> GHMGSSGGCTSMMNLVLCFTGFRKKEELVRLVTLVHHMGGVIRKDFNSKVTHLVANCTQGEKFRVAVSLGTPIMKPEWIYKAWERRNEQDFYAAVDDFRNEFKVPPFQDCILSFLGFSDEEKTNMEEMTEMQGGKYLPLGDERCTHLVVEENIVKDLPFEPSKKLYVVKQEWFWGSIQMDARAGETMYLYEKANTPELKKSVSMLSLNTPNSNRKRRRLKETLAQLSRETDVSPFPPRKRPSAEHSLSIGSLLDISNT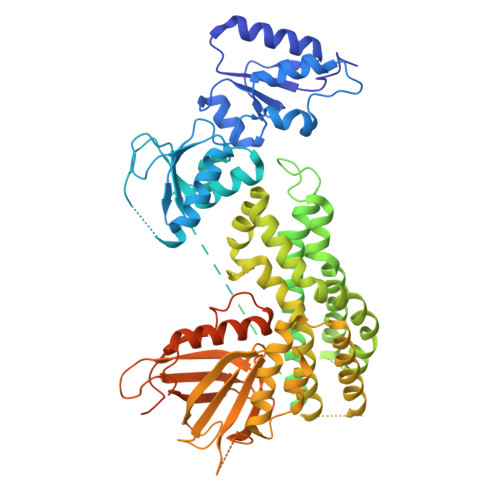PESSINYGDTPKSCTKSSKSSTPVPSKQSARWQVAKELYQTESNYVNILATIIQLFQVPLEEEGQRGGPILAPEEIKTIFGSIPDIFDVHTKIKDDLEDLIVNWDESKSIGDIFLKYSKDLVKTYPPFVNFFEMSKETIIKCEKQKPRFHAFLKINQAKPECGRQSLVELLIRPVQRLPSVALLLNDLKKHTADENPDKSTLEKAIGSLKEVMTHINEDKRKTEAQKQIFDVVYEVDGCPANLLSSHRSLVQRVETISLGEHPCDRGEQVTLFLFNDCLEIARKRHKVIGTFRSPHGQTRPPASLKHIHLMPLSQIKKVLDIRETEDCHNAFALLVRPPTEQANVLLSFQMTSDELPKENWLKMLCRHVANTICKADAENLIYTADPESFEVNTKDMDSTLSRASRAIKKTSKKVTRAFSFSKTPKRALRRALMTSHGSVEGRHHHHHH> GMGDAPSPEEKLHLITRNLQEVLGEEKLKEILKERELKIYWGTATTGKPHVAYFVPMSKIADFLKAGCEVTILFADLHAYLDNMKAPWELLELRVSYYENVIKAMLESIGVPLEKLKFIKGTDYQLSKEYTLDVYRLSSVVTQHDSKKAGAEVVKQVEHPLLSGLLYPGLQALDEEYLKVDAQFGGIDQRKIFTFAEKYLPALGYSKRVHLMNPMVPGLTGSKMSSSEEESKIDLLDRKEDVKKKLKKAFCEPGNVENNGVLSFIKHVLFPLKSEFVILRDEKWGGNKTYTAYVDLEKDFAAEVVHPGDLKNSVEVALNKL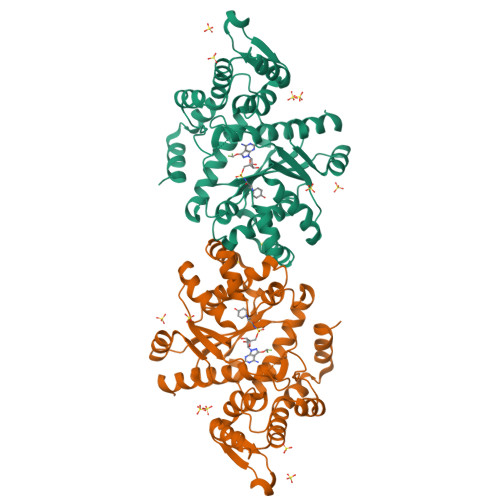LDPIREKFNTPALKKLASAAYPDPSKQKPMAKGPAKNSEPEEVI>MCTAITLNGNSNYFGRNLDLDFSYGEEVIITPAEYEFKFRKEKAIKNHKSLIGVGIVANDYPLYFDAINEDGLGMAGLNFPGNAYYSDALENDKDNITPFEFIPWILGQCSDVNEAR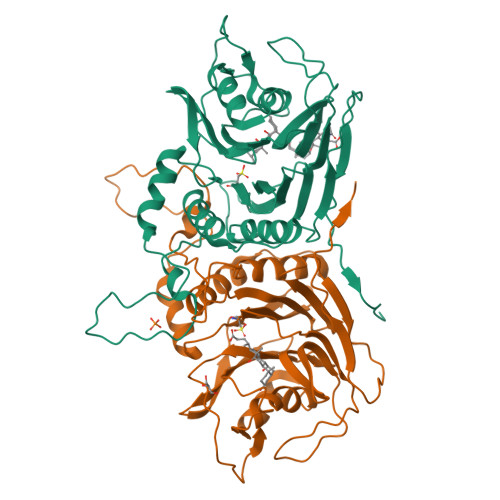NLVEKINLINLSFSEQLPLAGLHWLIADREKSIVVEVTKSGVHIYDNPIGILTNNPEFNYQMYNLNKYRNLSISTPQNTFSDSVDLKVDGTGFGGIGLPGDVSPESRFVRATFSKLNSSKGMTVEEDITQFFHILGTVEQIKGVNKTESGKEEYTVYSNCYDLDNKTLYYTTYENRQIVAVTLNKDKDGNRLVTYPFERKQIINKLNLERHHHHHH[8x]>KDRPDFCELPADTGPCRVRFPSFYYN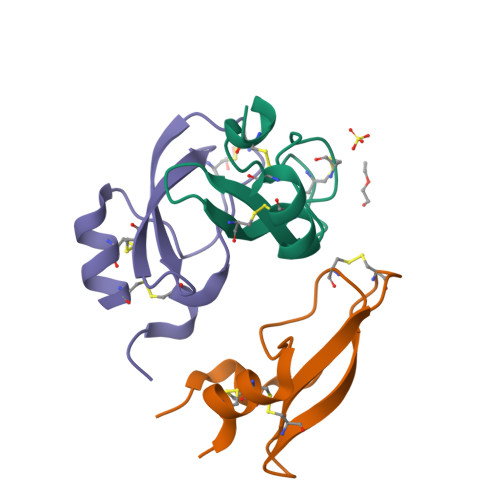PDEKKCLEFIYGGCEGNANNFITKEECESTCAA[3x]>MTDLKASSLRALKLMDLSTLNGDYTDEKVIALCH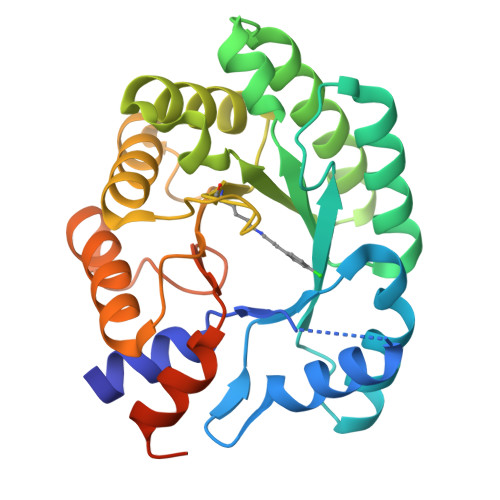QAKTPVGNTAAISVYPRSIPIARKTLKEQGTPEIRIATVTNFPHGNDDIEIALAETRAAIAYGADEVDVVFPYRALMAGNEQVGFDLVKACKEACAAANVLLKVIIETGELKDEALIRKASEISIKAGADFIKTSTGRVAVNATPESARIMMEVIRDMGVEKSVGFKVTGGVSTAEDAQKYLAIADELFGADWADARHYRFSASGLLASLLKALGHGDGKSASSYLEHHHHHH[2x]7-{3-(aminomethyl)-4-[(pyridin-2-yl)methoxy]phenyl}-4-methylquinolin-2-amine | C23 H22 N4 O 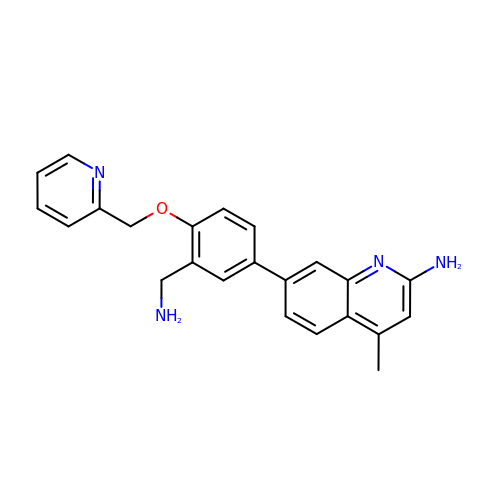| IYSGQZIVZRDDAE-UHFFFAOYSA-N>[2x]SVRKILRMGDPILRKISEPVTEDEIQTKEFKKLIRDMFDTMRHAEGVGLAAPQIGILKQIVVVGSEDNERYPGTPDV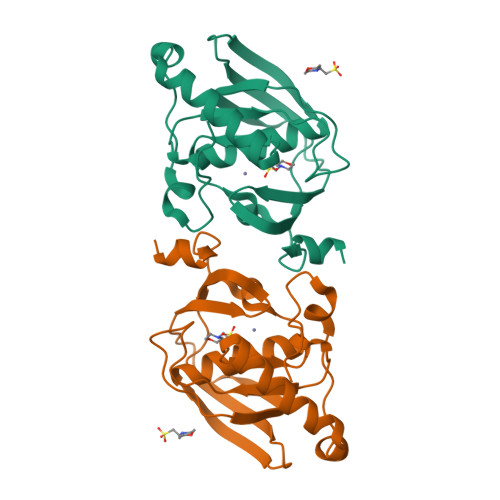PERIILNPVITPLTKDTSGFWEGCLSVPGMRGYVERPNQIRMQWMDEKGNQFDETIDGYKAIVYQHECDHLQGILYVDRLKDTKLFGFNETLDSSHNVLD2,4-dihydroxyphenacyl coenzyme 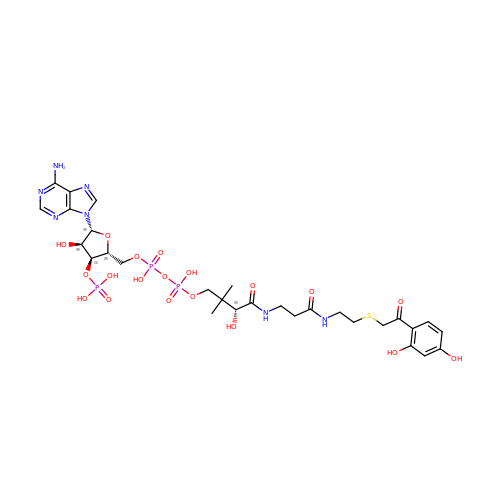A | C29 H42 N7 O19 P3 S | WNZSFAUZOOBNIR-VXAHOBLNSA-N> M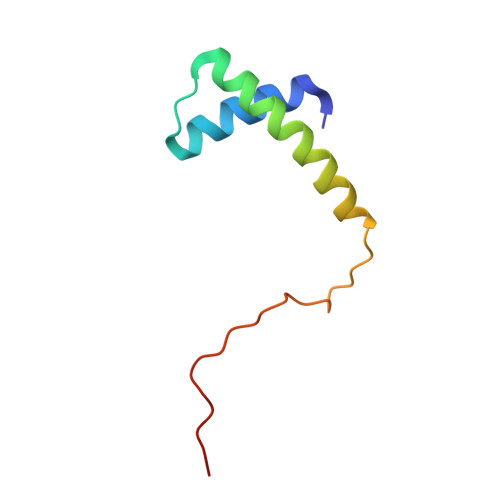TETEIFAYIEAASIAIGIPLEPARARAVAHHFSRTALLAEMLESVPLSPESELAEIYRPAPFPAEDI>[4x]MHHHHHHAMGNKIVFVEDDPEVGTLIAAYLGKHDMDVVVEPRGDRAEEVIAREKPDLVLLDIMLPGK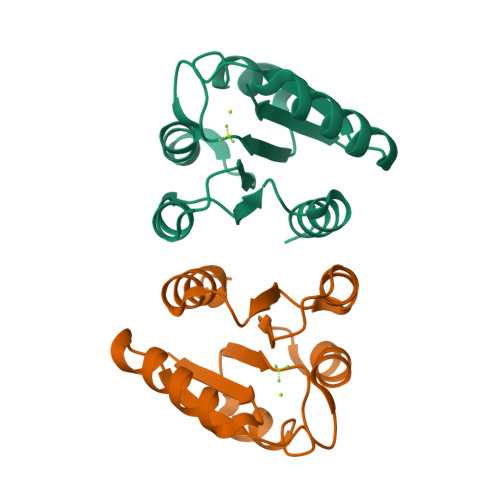DGMTLCRDLRGQWQGPIVLLTSLDSDMNHILSLEMGASDYILKTTPPAVLLARLRLHLRQH Bacteriophage Casadabanvirus JBD30, from the order Caudoviricetes, is a temperate phage that infects the bacterium Pseudomonas aeruginosa. The virion of bacteriophage JBD30 is composed of an icosahedral capsid, long flexible non-contractile tail, and a baseplate. Using its baseplate, JBD30 attaches to Pseudomonas aeruginosa via the bacterial type IV pilus, whose subsequent retraction brings the phage to the bacterial cell surface.

The stopper protein is composed of a four-stranded β-sheet and two α-helices connected by flexible loops. Each stopper protein (gp42) interacts with two adaptor proteins. The interactions between adaptor and stopper proteins are mainly electrostatic. Whereas the surface charge of the adaptor interface is positive, the interacting residues of the stopper protein are mostly negatively charged. Homologues of the stopper protein are found in the head-to-tail joining interface of the Rhodobacter capsulatus gene transfer agent, bacteriophage SPP1, and bacteriophage λ. Whereas the neck regions of bacteriophages SPP1 and λ are formed of three consecutive rings of adaptor, stopper, and tail-to-head joining proteins (gp15, gp16, gp17 for SPP1 and gpW, gpFII, gpU for phage λ), the neck of bacteriophage JBD30 has only adaptor and stopper proteins. The hexamer of stopper proteins provides an interface for tail attachment.

> MSDPFDYLFLEPLLIERIRSEVPGLAIVSGVPDLATLSEQDQPAPSAYVVYLGDETGTGADHQGGQRAIQTVGQQWAVVLVVHYADSSNSGEGARREAGPLLGRLVKALTGWAPAIDVAPLARSARQSPATYASGYLYFPLVFTARFVYPRIKSWKP1,2-DIMYRISTOYL-SN-GLYCERO-3-PHOSPHATE 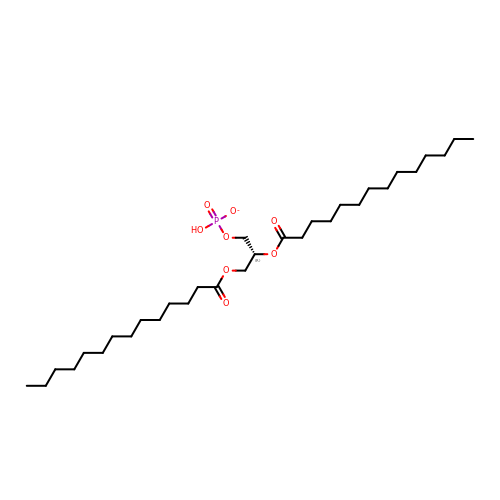| C31 H60 O8 P | OZSITQMWYBNPMW-GDLZYMKVSA-M> VGGESMLRGVYQDKFYQGTYPQNKNDNWLARATLIGK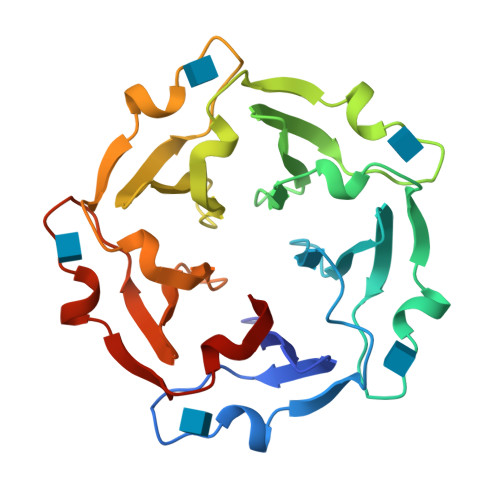GGWSNFKFLFLSPGGELYGVLNDKIYKGTPPTHDNDNWMGRAKKIGNGGWNQFQFLFFDPNGYLYAVSKDKLYKASPPQSDTDNWIARATEVGSGGWSGFKFLFFHPNGYLYAVHGQQFYKALPPVSNQDNWLARATKIGQGGWDTFKFLFFSSVGTLFGVQGGKFYEDYPPSYAYDNWLARAKLIGNGGWDDFRFLFF>[3x]MKLIVAIVRPEKLNEVLKALFQAEVRG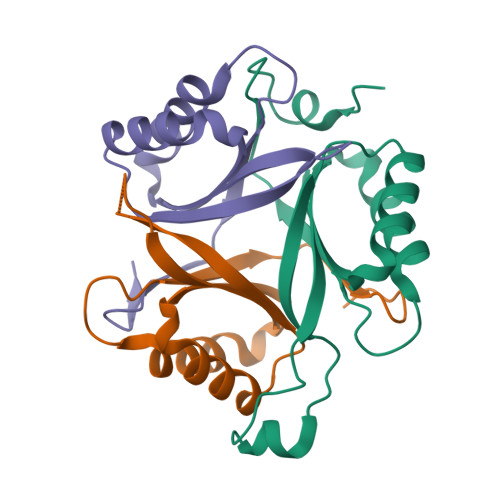LTLSRVQGHGGETERVETYRGTTVKMELHEKVRLEIGVSEPFVKPTVEAILKAARTGEVGDGKIFVLPVEKVYRIRTGEEDEAAVTPVQ> GSHMGGWSIALHGGAGDIPFSLPPERRKPREEGLRHCLQIGVEALKAQKPPLDVV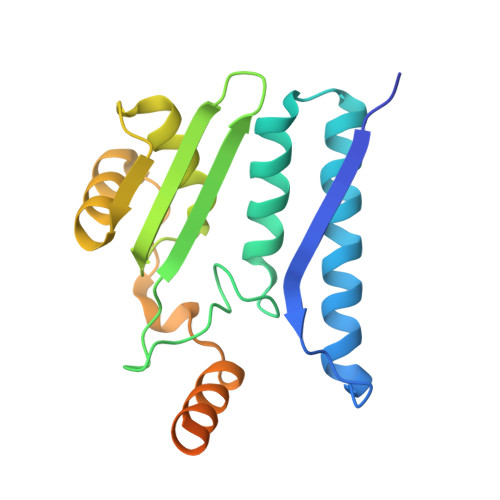ELVVRELENIEHFNAGIGSVLTNSGTVEMEASIMDGNTMKCGAVSGLSTVLNPISLARLVMDKTPHIYLAFQGAQDFAKQQGVETVDSSHLITAENVERLKLAIEANRVQVDYSQYNYPEPVKDDAEKELPLTNGDSQIG>[4x]GAMATSTAVFRIGLSDDVEFGLLPPLLRRLRAEAPGIVLVVRRANYLLMPNLLASGEISV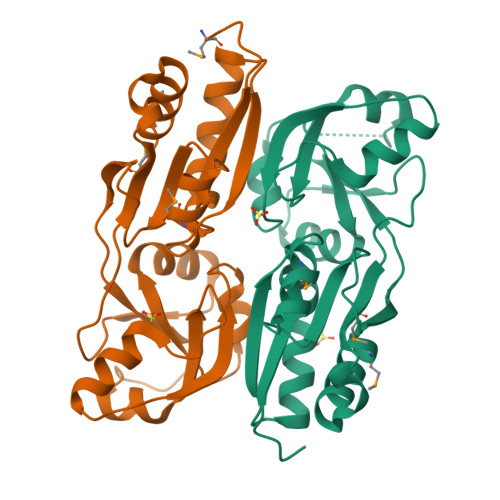GVSYTDELPANAKRKTVRRSKPKILRADSAPGQLTLDDYCARPHALVSFAGDLSGFVDEELEKFGRKRKVVLAVPQFNGLGTLLAGTDIIATVPDYAAQALIAAGGLRAEDPPFETRAFELSMAWRGAQDNDPAERWLRSRISMFIGDPDSL> ALRNGQYW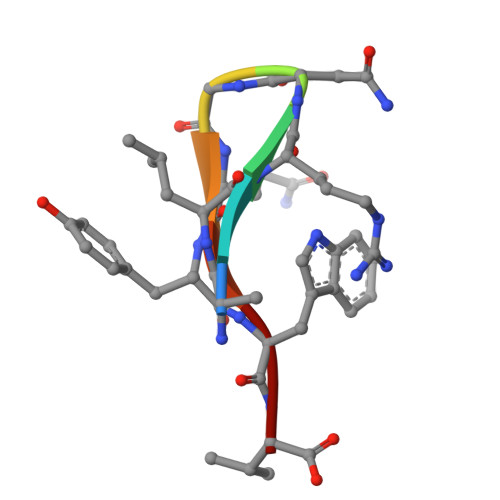V> SGDYWLPTTMSLYQKELTDQIVSLHYSDILRYFETSHYKEDVILESMKTMCLNGSLV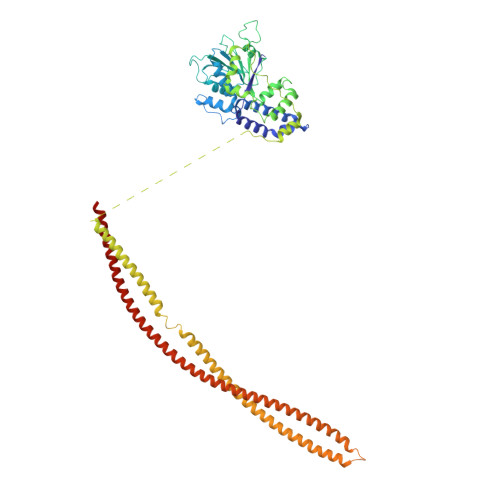ATHPYLLIDHYMPKSLITRDVPAHLAENSGKFSVLRDLINLVQEYETETAIVCRPGRTMDLLEALLLGNKVHIKRYDGHSIKSKQKANDFSCTVHLFSSEGINFTKYPIKSKARFDMLICLDTTVDTSQKDIQYLLQYKRERKGLERYAPIVRLVAINSIDHCRLFFGKKFDKNSREYLENVTAAMVILRDRLGTLPPDLRPIYSQKLHYLVEWLENPTVPWPLPDIYPLKQYTSMDVERSLLTEVHFKNSSNVNYHLSSGIITHKLIQSMGEVYMDICVQKQELDDYSCLDDLQNDHLKFFSNEDEKIIKEYETVLRTNNENLNRSHELEVENNLKFSQIETLEKDIETLKGSLMAQGETLSKLKDAFVKTDNVQDEIEKEERVSVSRDTEKKYMEQEIKRAVDAIRENEEETHKLNEKQNGLESELKLKFEKSEISTKELNEKIGFLKKELKLENDLNEELVGQLSKTMDNLENLTIPRVRTQ> AAAAAAAAAAAAAAAAAA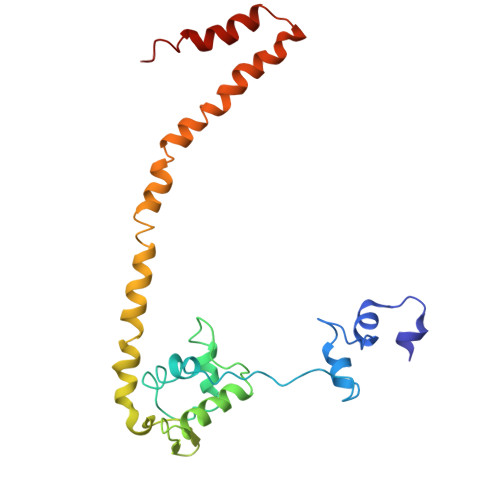AAAAAAAAAAAAAAAAAAAAAAAAAAAAAAAAAAAAAAAAAAAAAAAAAAAAAAAAAAAAAAAAAAAAAAAAAAAAAAAAAAAAAAAAAAAAAAAAAAAAAAAAAAAAAAAAAAAAAAAAAAAAAAAAAAAAAAAAAAAAAAAAAAAAAAAAAAAAAAAAAAAAAAAAAAAAAAAAAAAAAAAAA The first identified human member, ClC-1, is essential for maintaining the permeability of Cl− across the plasma membrane of skeletal muscle fibers, gCl, accounting for approximately 80% of the resting membrane conductance and assuring precise neuronal control of muscle contraction. Despite distinct roles as passively conducting Cl− channels and stoichiometrically coupled secondary active Cl−/H+ antiporters, members of the CLC family share a common homodimeric core architecture, with each subunit harboring an independent ion translocation pathway. In addition, the complex gating processes that regulate CLC channel activity remain elusive, with only a single available structure of a channel member, namely, that of bovine ClC-K. Each CLC monomer has a gate that operates independently from the other (also known as “protopore” or “fast gate”), structurally attributed to a specific glutamate, “GluGATE”. Here, we have determined structures of full-length human ClC-1 using single-particle cryo-electron microscopy (cryo-EM), exploiting a purified protein sample that displays Cl−-dependent single-channel–derived ion conductance.

For structural characterization, sample in the presence of 100 mM Cl− at pH 7.5 and in the absence of nucleotides or antibodies was initially employed. Three-dimensional (3D) classification of particles resulted in several different groups, of which one yielded a 3.6 Å overall resolution density map for the transmembrane domain, allowing confident model building. The final model represents the membrane-spanning portion (note that the N terminus and intracellular αA helix are lacking) as well as parts of two C terminal’s so-called cystathionine-β-synthase (CBS) domains present per monomer (for which some cryo-EM density is left unmodeled) and includes several features that were not observed in the ClC-K structure. In CLC transporters, the Cl− conducting pore is marked by distinct Cl− binding sites (denoted sext, scen, and sint, respectively, but no Cl− ions are resolved in the current structure), and the constricting Glu232 (of αF, also known as GluGATE; ClC-1 numbering throughout) and Tyr578 (of αR, TyrC). Unfortunately, the GluGATE side chain is not visible in our cryo-EM density maps, but carboxylate groups of interacting acidic residues are known to be frequently undetectable using cryo-EM due to radiation damage. The pore aperture of the extracellular vestibule is constricted by a hydrophobic barrier with Met485 (Met427 in ClC-K), but in contrast to ClC-K, the gate opening is also controlled by Lys231 (of αE–F) and Arg421 (of αL) that may orchestrate Cl− permeation to or from the extracellular environment. This difference can be attributed to αE–F, with its GluGATE and Lys231 adopting a more CLC-transporter–like configuration because this loop is considerably shorter than in ClC-K, alongside a side-chain reorientation of Arg421.

>[2x]MEQSRSQQRGGEQSWWGSDPQYQYMPFEHCTSYGLPSENGGLQHRLRKDAGPRHNVHPTQIYGHHKEQFSDREQDIGMPKKTGSSSTVDSKDEDHYSKCQDCIHRLGQVVRRKLGEDGIFLVLLGLLMALVSWSMDYVSAKSLQAYKWSYAQMQPSLPLQFLVWVTFPLVLILFSALFCHLISPQAVGSGIPEMKTILRGVVLKEYLTMKAFVAKVVALTAGLGSGIPVGKEGPFVHIASICAAVLSKFMSVFCGVYEQPYYYSDILTVGCAVGVGCCFGTPLGGVLFSIEVTSTYFAVRNYWRGFFAATFSAFVFRVLAVWNKDAVTITALFRTNFRMDFPFDLKELPAFAAIGICCGLLGAVFVYLHRQVMLGVRKHKALSQFLAKHRLLYPGIVTFVIASFTFPPGMGQFMAGELMPREAISTLFDNNTWVKHAGDPESLGQSAVWIHPRVNVVIIIFLFFVMKFWMSIVATTMPIPCGGFMPVFVLGAAFGRLVGEIMAMLFPDGILFDDIIYKILPGGYAVIGAAALTGAVSHTVSTAVICFELTGQIAHILPMMVAVILANMVAQSLQPSLYDSIIQVKKLPYLPDLGWNQLSKYTIFVEDIMVRDVKFVSASYTYGELRTLLQTTTVKTLPLVDSKDSMILLGSVERSELQALLQRHLCPERRLRAAQEMARKLSELPYDGKARLAGEGLPGAPPGRPESFAFVDEDEDEDLSGKSELPPSLALHPSTTAPLSPEEPNGPLPGHKQQPEAPEPAGQRPSIFQSLLHCLLGRARPTKKKTTQDSTDLVDNMSPEEIEAWEQEQLSQPVCFDSCCIDQSPFQLVEQTTLHKTHTLFSLLGLHLAYVTSMGKLRGVLALEELQKAIEGHTKSGVQLRPPLASFRNTTSTRKSTGAPPSSAENWNLPEDRPGATGTGDVIAASPETPVPSPSPEPPLSLAPGKVEGELEELELVESPGLEEELADILQGPSLRSTDEEDEDELIL> APSKVQRAPDSSIHARAVCTPTAGGDSSTDDVPAITEALSSCGNGGTIVFPEGSTYYLNSVLDLGSCSDCDIQVEGLLKFASDTDYWSGRTAMISVSNVDGLKLRSLTGSGVIDGNGQDAWDLFASDSSYSRPTLLYITGGSNLEISGLRQKNPPNVFNSVKGGATNVVFSNLKMDANSKSDNPPKNTDGFDIGESTYVTITEVTVVNDDDCVAFKPSSNYVTVDTISCTGSHGISVGSLGKSSDDSVKNIYVTGATMINSTKAAGIKTYPSGGDHGTSTVSNVTFNDFTVDNSDYAFQ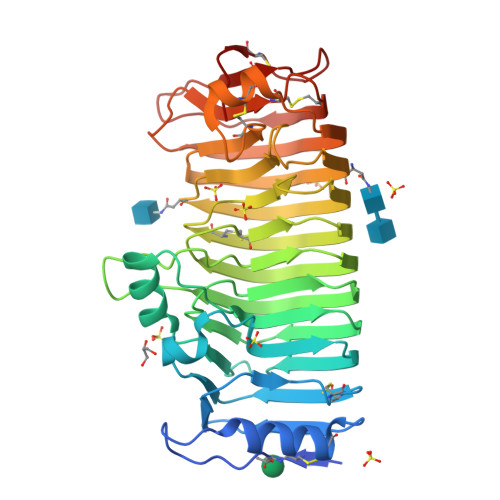IQSCYGEDDDYCEENPGNAKLTDIVVSSFSGTTSDKYDPVVANLDCGADGTCGISISGFDVKAPSGKSEVLCANTPSDLGVTCTSGASG>[2x]T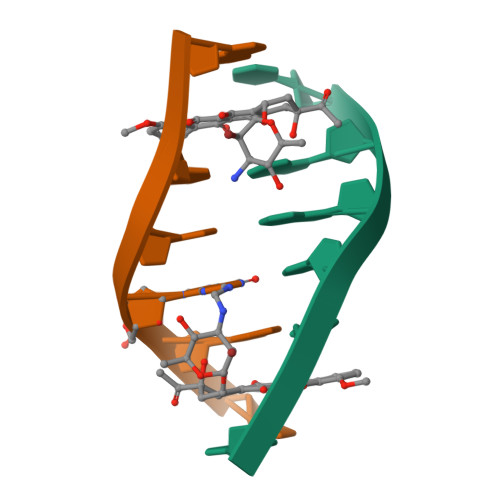GGCCG E. coli NfsB belongs to an extensive, functionally diverse nitroreductase superfamily, members of which are united by a conserved structural fold and fundamental mechanism of catalysis. NfsB family nitroreductases catalyze the reduction of nitroaromatic compounds, a step that is pivotal in various biochemical processes and exploited for bioremediation and cancer therapies. This catalytic mechanism involves hydride transfer from a reduced cofactor, such as reduced nicotinamide adenine dinucleotide (phosphate) (NAD(P)H), to the nitro group of the substrate, leading to its conversion via a nitroso intermediate into the corresponding hydroxylamine or amine. The reductive half reaction consists of initial hydride transfer from NAD(P)H to a bound flavin mononucleotide (FMN) moiety, and the oxidative half reaction consists of subsequent hydride transfer from the reduced FMN to an electron acceptor substrate (e.g., the nitro group of an aromatic ring).

Here, we describe our solution of the E. coli NfsB F70A/F108Y structure to 1.98 angstroms and comparative modeling of each of SN33623, CB1954, and metronidazole in the active sites of the parental and F70A/F108Y enzymes. The biological assembly of E. coli NfsB F70A/F108Y is a homodimer of two 24 kDa subunits, where each monomer exhibits the conserved α+β fold and FMN binding residues characteristic of members of the nitroreductase superfamily. Each dimer has two FMN binding sites, located at the interface, and contributed to by residues from both monomers. Electron density was found to accommodate one molecule of acetate at the re-face of the FMN in each active site of the crystal structure. Acetate was present in the crystallization buffer and has been reported to act as a competitive inhibitor to nitroreductases. The structure of the mutant and the parental enzyme are largely identical (RMSD of Cα atoms between the two structures is 0.32 Å), however some significant conformational changes were noted in the active site. First, the aromatic ring at position F70 is absent in the double mutant. Second, the side chain of N67 adopts an alternate conformation in the double-mutant structure, effectively widening the entrance of the active site’s entrance channel. Third, in the double-mutant active site, we observe the side chain hydroxyl group of Y108 participates in direct hydrogen bonding to the carboxamide/carboxyl groups of N117 and E102, respectively. Fourth, the aromatic rings at positions F123 and F124 are displaced in the double-mutant structure compared with the wild type and their average B-factors are higher, suggesting greater flexibility.

>[4x]MDIISVALKRHSTKAFDASKKLTPEQAEQIKTLLQYSPSSTNSQPWHFIVASTEEGKARVAKSAAGNYVANERKMLDASHVVVFCAKTAMDDVWLKLVVDQEDADGRYATPEAKAANDKGRKFFADMHRKDLHDDAEWMAKQVYLNVGNFLLGVAALGLDAVPIEGFDAAILDAEFGLKEKGYTSLVVVPVGHHSVEDFNATLPKSRLPQNITLTEV> GPRSRLLLGPNSASSSTKLDDDLGTAAAVLSNMRSSPYRTHDKP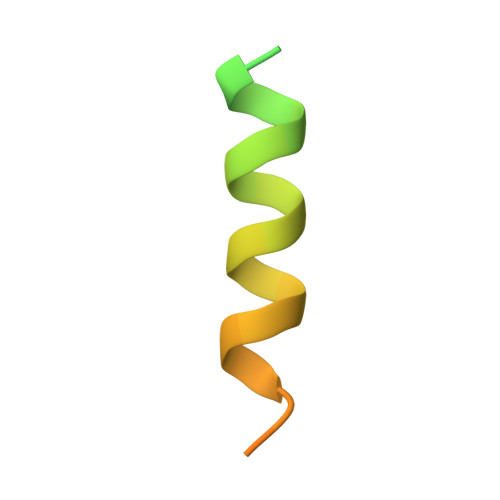IS>[2x]LKCHNKLVPFLSKTCPEGKNLCYKMTLMKMPKIPIKRGCTDACPKSSLLVKVVCCNKDKCN

3FTxs, non-enzymatic snake venom proteins, are the most abundant toxins found in elapid (cobras, kraits, mambas and sea snakes) and colubrid venoms. Structurally, all 3FTxs have a stable fold with three β-stranded loops extending from a central core containing all four conserved disulphide bridges, resembling the three fingers of a hand, and hence their common name. Despite overall similar fold, 3FTxs recognize a broad range of distinct molecular targets resulting in diverse biological activities. In continuation of our efforts to understand the relationship between the structure and function of 3FTxs, we isolated, purified and determined the complete amino acid sequence and the crystal structure of a new three-finger toxin (hemachatoxin) from H. haemachatus (Ringhals cobra) venom at 2.43 Å resolution.

There were two hemachatoxin molecules in an asymmetric unit with each molecule consisting of residues from Leu1 to Asn61. Each monomer of the asymmetric unit consists of 6 anti-parallel β-strands (β2↓β1↑β4↓β3↑β6↓β5↑) that form two β-sheets. The first β-sheet consists of two anti-parallel β-strands, β1 (Lys2-Lys6) and β2 (Phe10-Thr14), while the second contains four anti-parallel strands, β3 (Leu21-Thr26), β4 (Ile35-Thr40), β5 (Ala42-Ser47) and β6 (Lys51-Asn56). The fold of hemachatoxin is maintained by four disulfide bonds, and these cysteines are strictly conserved among the 3FTxs. The electrostatic surface representation shows that loops I and II are predominantly charged residues, whereas loop III is highly hydrophobic in nature. ESI-MS, Edman degradation and crystal structure data indicates that hemachatoxin differs from cytotoxin 1 in two amino acid positions (Leu27Met28 is replaced by Met27Leu28) and hence are isoforms. Hemachatoxin shows highest similarity to P-type cardiotoxins. Similar to these P-type cardiotoxins, hemachatoxin has the conserved Pro31 and cytolytic site. The three-dimensional structure is similar to P-type cardiotoxins (RMSD values, 0.8 to 2.1 Å for 58 to 60 Cα atoms; Z score values, 12.2 to 9.8). Nonetheless this analysis suggests that loop II is flexible and may remain flexible until its interaction with membrane phospholipids.> KWKWWEEERYPEGIKWKFLEHKGPVFAPPYEPLPENVKFYYDGKVMKLSPKAEEVATFFAKMLDHEYTTKEIFRKNFFKDWRKEMTNEEKNIITNLSKCDFTQMSQYFKAQTEARKQMSKEEKLKIKEENEKLLKEYGFCIMDNHKERIANFKIEPPGLFRGRGNHPKMGMLKRRIMPEDIIINCSKDAKVPSPPPGHKWKEVRHDNKVTWLVSWTENIQGSIKYIMLNPSSRIKGEKDWQKYETARRLKKCVDKIRNQYREDWKSKEMKVRQRAVALYFIDKLALRAGNEKEEGETADTVGCCSLRVEHINLHPELDGQEYVVEFDFLGKDSIRYYNKVPVEKRVFKNLQLFMENKQPEDDLFDRLNTGILNKHLQDLMEGLTAKVFRTYNASITLQQQLKELTAPDENIPAKILSYNRANRAVAILCNHQRAPP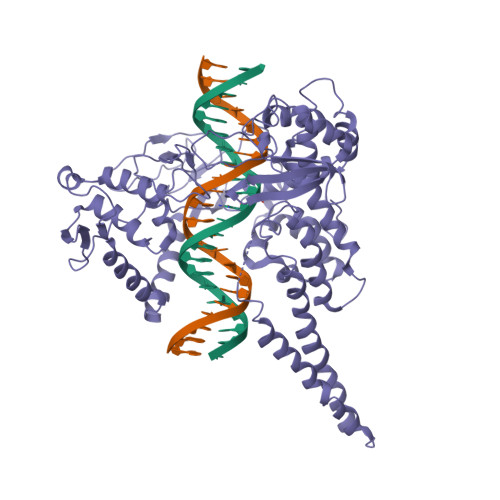KTFEKSMMNLQTKIDAKKEQLADARRDLKSAKADAKVMKDAKTKKVVESKKKAVQRLEEQLMKLEVQATDREENKQIALGTSKLNFLDPRITVAWCKKWGVPIEKIYNKTQREKFAWAIDMADEDYEF> MVCCLWVLLALLLHLDHVACEDDAYSFTSKELKAYKQEVKELFYFGFDNYLEHGYPYDEVKPISCVPKKRNFEDPTDQGTNDILGNFTITLIDSLTTIAILEDRPQFLKAVRLVERTFPDGNFDIDSTIQVFEITIRVIGSLLSSHLYATDPTKAVYLGDDYDGSLLRLAQNMADRLLPAYLTSTGLPMPRRNIKRKWDVSEFPEFLETENNVAAMASPMFEFTILSYLTGDPKYEKVTRYAFDKTWSLRTGLDLLPMSFHPEKLTPYTPMTGIGASIDSLFEYALKGAILFDDSELMEVWNVAYEALKTNCKNDWFFANVMADTGHLFVPWIDSLSAFFSGLQVLAGDLDDAIANHLMFLKMWNTFGGIPERWNFSPPEFPPLSPLERSGAVALDNILPLEWYPLRPEFFESTYFLYRATKDPFYLNIGVHLLKDLKQRFKSNCGFAGFQNVITGELQDRMETFVLSETLKYLYLLFDEENELHNSASDVIFSTEAHPMWLPQEVRSNYKRNAKFNNSVYSSHLEICQKKDREQAGENTLSQRIVGFAKSIFHKGPPDEEATDPIIDYTIDTELPGTCSIKPHHVIGDEFWYSPMLSNFDRLFEIDSRFAATLIKPSHMHNYNAIELEPGFYNRWSNPQFSTCLIPPTTEIFELLFDLPGYHQLNPLMLENKTITFETFGGRSRLKIEKLQIYQIDYYGDLITASTFQDVSRKDIFSNACDAVASLYSPTYLYRVVAINGRILPRHGSVQIKKHSPVLTSNGTREEDEFKMDGIGINDHSQLMLECTPIINLFIV;> MKFSAGAVLSWSSLLLASSVFAQQEAVAPEDSAVVKLATDSFNEYIQSHDLVLAEFFAPWCGHCKNMAPEYVKAAETLVEKNITLAQIDCTENQDLCMEHNIPGFPSLKIFKNSDVNNSIDYEGPRTAEAIVQFMIKQSQPAVAVVADLPAYLANETFVTPVIVQSGKIDADFNATFYSMANKHFNDYDFVSAENADDDFKLSIYLPSAMDEPVVYNGKKADIADADVFEKWLQVEALPYFGEIDGSVFAQYVESGLPLGYLFYNDEEELEEYKPLFTELAKKNRGLMNFVSIDARKFGRHAGNLNMKEQFPLFAIHDMTEDLKYGLPQLSEEAFDELSDKIVLESKAIESLVKDFLKGDASPIVKSQEIFENQDSSVFQLVGKNHDEIVNDPKKDVLVLYYAPWCGHCKRLAPTYQELADTYANATSDVLIAKLDHTENDVRGVVIEGYPTIVLYPGGKKSESVVYQGSRSLDSLFDFIKENGHFDVDGKALYEEAQEKAAEEADADAELADEEDAIHDEL

In Saccharomyces cerevisiae, the glycan of these proteins is trimmed by the luminal mannosidase Mnl1 (Htm1) to generate a degradation signal. Curiously, Mnl1 forms a permanent complex with protein disulfide isomerase (Pdi1), a redox enzyme found in all eukaryotic cells. Here, we show that the Mnl1–Pdi1 complex initiates ERAD-L by performing two crucial reactions on glycoprotein substrates, trimming the glycan and reducing disulfide bonds. Pdi1 contains four thioredoxin-like (Trx) domains (a, b, b′ and a′), with a and a′ containing redox-active CGHC motifs.

A cryo-EM structure of the Mnl1–Pdi1 complex was obtained from a particle class after three-dimensional (3D) classification and refinement and had an overall resolution of 3.0 Å. The density map of this class (complete) allowed model building for most parts of the proteins (examples in Extended Data Fig. 3), with the exception of some Mnl1 loops. The density of a C-terminal domain (CTD) was weaker than that for other parts of the protein. Mnl1 consists of a canonical mannosidase domain (MHD; amino acids 29–514), a loop interacting with Pdi1 (residues 515–650) and the CTD (residues 651–796). The MHD forms a barrel with a central pore. The CTD interacts weakly with one side of the mannosidase barrel. The Mnl1 loop interacts with domains a, b′ and a′. The total interaction surface is fairly large (2,480 Å2). The Mnl1 loop contains two cysteines (C579 and C644) that are in disulfide-bonding distance to the first cysteines of the redox-active CGHC motifs of the a′ and a Trx domains of Pdi1.>GSFNSLEACLPATCLEPCVICQSRPKNGCIVHGRTGHLMACYTCAKKLKNRNKLCP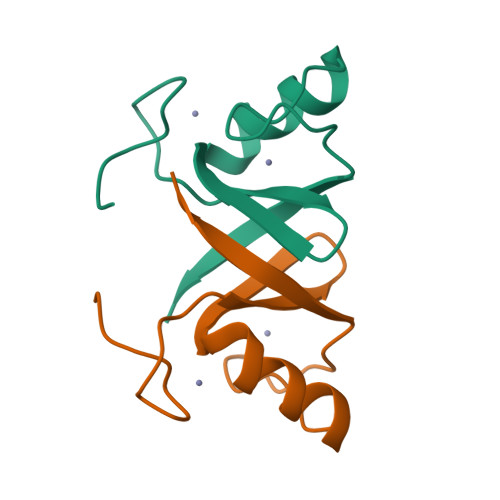VCREPIQSVVLTYMS[2x]> KETAAAKFER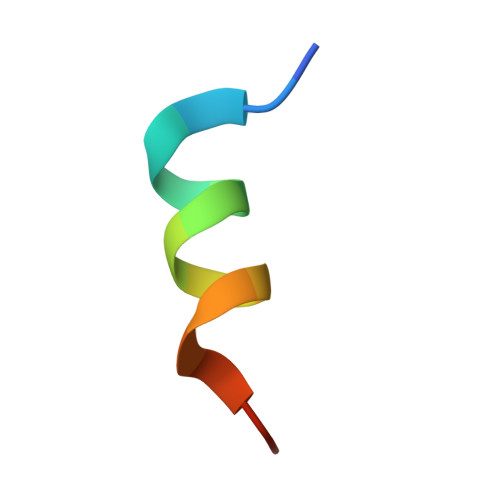QHADSX>[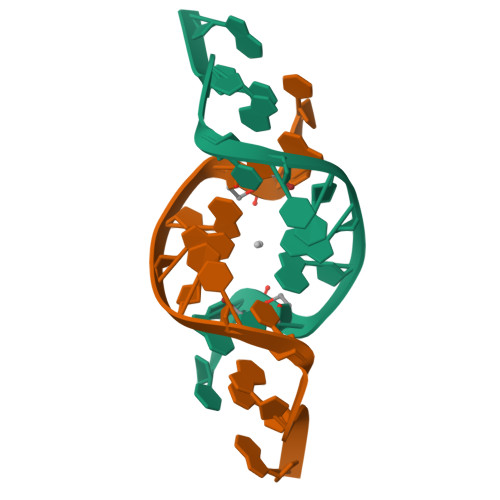2x]CGCGANTCGCG>EWTGDNTNAYYSDEVISELHVGQIDTSPYFCIKTVKANGSGTPVVACAVSKQSIWAPSFKELLDQARYFYSTGQSVRIHVQKNIWTYPLFVNTFSANALVGLSSCSATQCFGPKLEHH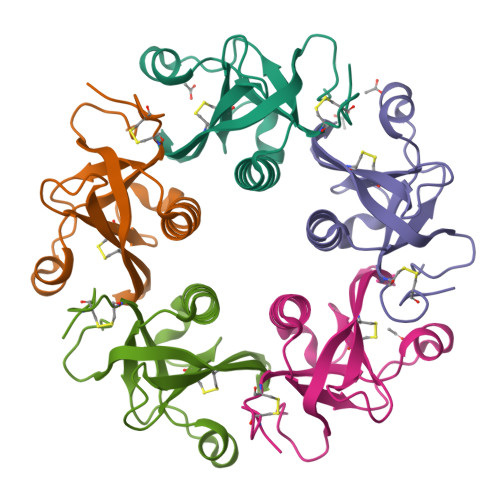HHHH[5x]>MKIQMRNKKVLSFLTLTAIVSQALVYPVYAQTSTSNHSNKKKEIVNEDILPNNGLMGYYFTDEHFKDLKLMAPIKDGNLKFEEKKVDKLLDKDKSDVKSIRWTGRIIPSKDGEYTLSTDRDDVLMQVNTESTISNTLKVNMKKGKEYKVRIELQDKNLGSIDNLSSPNLYWELDGMKKIIPEENLFLRDYSNIEKDDPFIPNNNFFDPKLMSDWEDEDLDTDNDNIPDSYERNGYTIKDLIAVKWEDSFAEQGYKKYVSNYLESNTAGDPYTDYEKASGSFDKAIKTEARDPLVAAYPIVGVGMEKLIISTNEHASTDQGKTVSRATTNSKTESNTAGVSVNVGYQNGFTANVTTNYSHTTDNSTAVQDSNGESWNTGLSINKGESAYINANVRYYNTGTAPMYKVTPTTNLVLDGDTLSTIKAQENQIGNNLSPGDTYPKKGLSPLALNTMDQFSSRLIPINYDQLKKLDAGKQIKLETTQVSGNFGTKNSSGQIVTEGNSWSDYISQIDSISASIILDTENESYERRVTAKNLQDPEDKTPELTIGEAIEKAFGATKKDGLLYFNDIPIDESCVELIFDDNTANKIKDSLKTLSDKKIYNVKLERGMNILIKTPTYFTNFDDYNNYPSTWSNVNTTNQDGLQGSANKLNGETKIKIPMSELKPYKRYVFSGYSKDPLTSNSIIVKIKAKEEKTDYLVPEQGYTKFSYEFETTEKDSSNIEITLIGSGTTYLDNLSITELNSTPEILDEPEVKIPTDQEIMDAHKIYFADLNFNPSTGNTYINGMYFAPTQTNKEALDYIQKYRVEATLQYSGFKDIGTKDKEMRNYLGDPNQPKTNYVNLRSYFTGGENIMTYKKLRIYAITPDDRELLVLSVD[3x];> YSEKVCNTTYKAPIERPEDFLKDKEKAKEWERKEAERIEQKLERSEKEALESYKKDSVEISKYSQTRNYFYDYQIEANSREKEYKELRNAISKNKIDKPMYVYYFESPEKFAFNKVIRTENQNEISLEKFNEFKETIQNKLFKQDGFKDISLYEPGKGDEKPTPLLMHLKLPRNTGMLPYTNTNNVSTLIEQGYSIKIDKIVRIVIDGKHYIKAEASVVSSLDFKDDVSKGDSWGKANYNDWSNKLTPNELADVNDYMRGGYTAINNYLISNGPVNNPNPELDSKITNIENALKREPIPTNLTVYRRSGPQEFGLTLTSPEYDFNKLENIDAFKSKWEGQALSYPNFISTSIGSVNMSAFAKRKIVLRITIPKGSPGAYLSAIPGYAGEYEVLLNHGSKFKINKIDSYKDGTITKLIVDATLIP

CDT is a member of the Iota family of protein toxins which also consists of two homologous toxins produced by Clostridium perfringens (the Iota toxin) and Clostridium spiroforme (C. spiroforme Transferase, CST). All three Iota toxin family members are assembled from two polypeptide chains termed the “A” subunit (CDTa, Ia, and CSTa) and “B”, subunit (CDTb, Ib, and CSTb). All three B subunits are presumed to contain five domains that are involved in regulation (D1), oligomerization (D2 and D3), and host recognition (D3’ and D4). Once proteolyzed, the mature form of CDTb forms a large heptameric, soluble structure referred to as the prepore which binds one molecule of CDTa to generate the toxic moiety, CDT.

We also uncovered a subpopulation of the CDTb trimer bound to CDTa but note that these particles are present in a significantly lower abundance, indicating the CDTa bound dimer is preferred. Still, we were able to generate a low-resolution map (8.15 Å) and assemble a model of the CDTb trimer bound to CDTa. The resulting structure illustrates rotations of Chains B and C of ~4° and ~9° about the central pseudosymmetry axis when compared to the apo structure, respectively, that allows for interactions with CDTa in both chains. This results in an orientation of Chain C that closely resembles CDTb protomers as they are arranged in the symmetric heptamer. (G) The relative orientations of Chains B and C within the trimeric intermediate shift to contact CDTa, resulting in a structure that resembles that of the assembled, symmetric prepore. Similarly, the reorientation of CDTb protomers in the assembly intermediates bound to CDTa suggests that CDTa may also induce toxin assembly through the stabilization of the heptameric form of CDTb.> MQAQQLPYEFFSEENAPKWRGLLVPALKKVQGQVHPTLESNDDALQYVEELILQLLNMLCQAQPRSASDVEERVQKSFPHPIDKWAIADAQSAIEKRKRRNPLSLPVEKIHPLLKEVLGYKIDHQVSVYIVAVLEYISADILKLVGNYVRNIRHYEITKQDIKVAMCADKVLMDMFHQDVEDINILSLTDEEPSTSGEQTYYDLVKAFMAEIRQYIRELNLIIKVFREPFVSNSKLFSANDV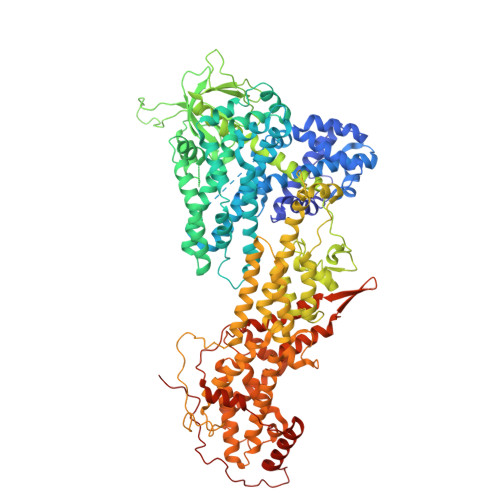ENIFSRIVDIHELSVKLLGHIEDTVEMTDEGSPHPLVGSCFEDLAEELAFDPYESYARDILRPGFHDRFLSQLSKPGAALYLQSIGEGFKEAVQYVLPRLLLAPVYHCLHYFELLKQLEEKSEDQEDKECLKQAITALLNVQSGMEKICSKSLAKRRLSESACRFYSQQMKGKQLAIKKMNEIQKNIDGWEGKDIGQCCNEFIMEGTLTRVGAKHERHIFLFDGLMICCKSNHGQPRLPGASNAEYRLKEKFFMRKVQINDKDDTNEYKHAFEIILKDENSVIFSAKSAEEKNNWMAALISLQYRSTLERMLDVTMLQEEKEEQMRLPSADVYRFAEPDSEENIIFEENMQPKAGIPIIKAGTVIKLIERLTYHMYADPNFVRTFLTTYRSFCKPQELLSLIIERFEIPEPEPTEADRIAIENGDQPLSAELKRFRKEYIQPVQLRVLNVCRHWVEHHFYDFERDAYLLQRMEEFIGTVRGKAMKKWVESITKIIQRKKIARDNGPGHNITFQSSPPTVEWHISRPGHIETFDLLTLHPIEIARQLTLLESDLYRAVQPSELVGSVWTKEDKEINSPNLLKMIRHTTNLTLWFEKCIVETENLEERVAVVSRIIEILQVFQELNNFNGVLEVVSAMNSSPVYRLDHTFEQIPSRQKKILEEAHELSEDHYKKYLAKLRSINPPCVPFFGIYLTNILKTEEGNPEVLKRHGKELINFSKRRKVAEITGEIQQYQNQPYCLRVESDIKRFFENLNPMGNSMEKEFTDYLFNKSLEIEPRNPKPLPRFPKKYSYPLKSPGVRPSNPRPGT>[4x]GSHMEEGGTRNREEGKMKETTIVVYERPDIYDPIFIEGLPGIGLVGKLAAEHLIQELKAKKFAELYSPHFMHQVLIRKNSVVELMKNEFYYWKSPDDEHRDLIIVTGDTQVPPTDSYGHFEVAGKMLDFVQEFGTREIITMGGYQVPEIQGEPRVLAAVTHEDLIEYYKSKLEGCS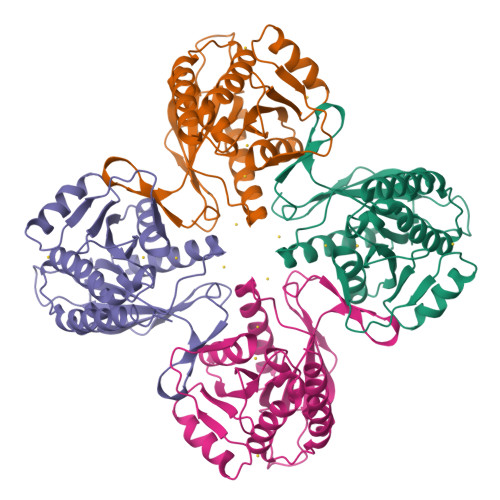VEVIWREDEGGAIVGAAGLLLGIGKLRGMFGISLLGESLGYIVDAKAAKAVLSAVTKILGLEIDMTALDERAKETEEILRKVEEMQRAMMEQVTPKLPHEEEDRGYL> MTNPSNSNLQALREELCTPGLDQGHLFEGWPETVDECNERQIALLTDLYMFSNMYPGGVAQYIRNGHELLARESEEVDFAALEMPPLIFEAPSLHRRTAERTALENAGTAMLCKTVFVLVAGGLGERLGYSSIKVSLPVETATNTTYLAYYLRWAQRVGGKEVPFVIMTSDDTHDRTLQLLRELQLEVPNLHVLKQGQVFCFADSAAHLALDETGKLLRKPHGHGDVHSLIYNATVKRDVVPDSGDGTATAQPLVNDWLAAGYESIVFIQDTNAGATITIPISLALSAEHSLDMNFTCIPRVPKEPIGLLCRTKKNSGDPWLVANVEYNVFA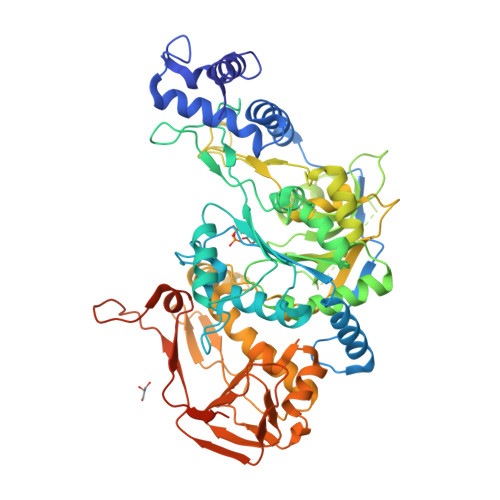EVSRALNKDGGDEVSDPTGFSPFPGSVNTLVFKLSSYVDRLRESHGIVPEFINPKYSDETRRSFKKPARIESLMQDIALLFSEDDYRVGGTVFERFSYQPVKNSLEEAAGLVAQGNGAYCAATGEAAFYELQRRRLKAIGLPLFYSSQPEVTVAKDAFGVRLFPIIVLDTVCASSGSLDDLARVFPTPEKVHIDQHSTLIVEGRVIIESLELYGALTIRGPTDSMALPHVVRNAVVRNAGWSVHAILSLCAGRDSRLSEVDRIRGFVLKKTAMAVMDCNTKGESEAGAPSGAADPAKLMRRLEHHHHHH>[4x]MSVNLASQLRE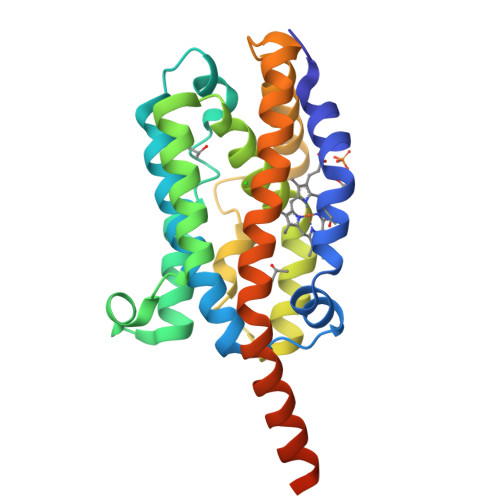GTKKSHSMAENVGFVKCFLKGVVEKNSYRKLVGNLYFVYSAMEEEMAKFKDHPILSHIYFPELNRKQSLEQDLQFYYGSNWRQEVKISAAGQAYVDRVRQVAATAPELLVAHSYTRYLGDLSGGQILKKIAQNAMNLHDGGTAFYEFADIDDEKAFKNTYRQAMNDLPIDQATAERIVDEANDAFAMNMKMFNELEGNLIKAIGIMVFNSLTRRRSQGSTEVGLATSEG> MKKSKRKNAQAQEAQETEVLVQEEAEELPEFP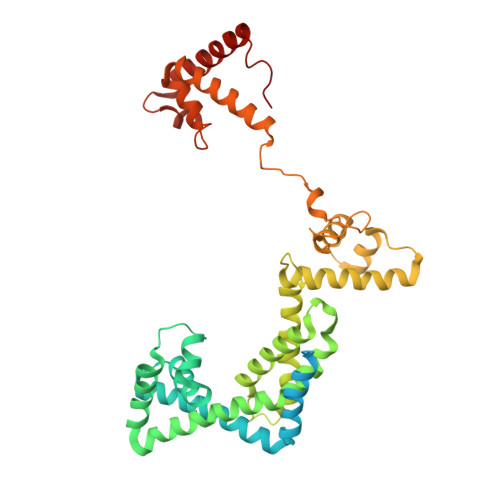EGEPDPDLEDPDLALEDDLLDLPEEGEGLDLEEEEEDLPIPKISTSDPVRQYLHEIGQVPLLTLEEEVELARKVEEGMEAIKKLSEITGLDPDLIREVVRAKILGSARVRHIPGLKETLDPKTVEEIDQKLKSLPKEHKRYLHIAREGEAARQHLIEANLRLVVSIAKKYTGRGLSFLDLIQEGNQGLIRAVEKFEYKRRFKFSTYATWWIRQAINRAIADQARTIRIPVHMVETINKLSRTARQLQQELGREPTYEEIAEAMGPGWDAKRVEETLKIAQEPVSLETPIGDEKDSFYGDFIPDEHLPSPVDAATQSLLSEELEKALSKLSEREAMVLKLRKGLIDGREHTLEEVGAFFGVTRERIRQIENKALRKLKYHESRTRKLRDFLD> MLSVSPPLRRYRLFHPRREAIPMHMCPAKTIFPLINSNNLLVKTRNSWEDFTGRKEFDEDHPLPVVGSRLNGRTTQHKWNHWDQYLNPQITQSIKDLTPTPEYVGMRCGHNMIKMGWMKIGGSWKYSRGYNDRRRVFARGQWQERKMTP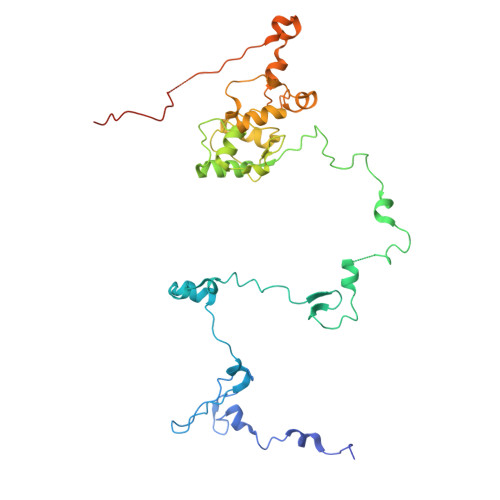RFMLAPRVSAGGPRNRYEGKLVFSPLRLSKLLWAIDTGRINPNEVITLYHLRQANVVGEREIVWPGFVLISNGVRRVPYPIHIELQNASAESIRLIEEAGGSFTCVYMTHEGLYQELHPEEYPIFMDQELPERRGLESLATNPSKRGWLTRWYEDSSKYAHPAAGRRYSHYLKPPTERDFPATVEEYEMVKHHQKWHLNQPGTGTLLPWHSYNTADLVKRAAGRL>[4x]RHMQEILDAILSGDAASADYAALALPESYRAVTLHKGEERMFDGLASRDKDPRKSLHLDDVPLPELGPGEALVAVMASSVN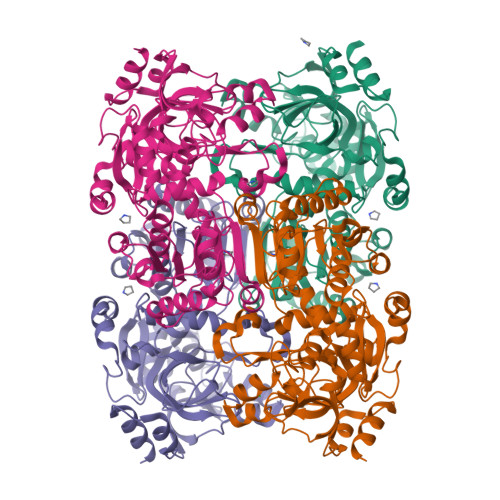YNTVWSSIFEPVSTFGFLERYGRLSPLTARHDLPYHVLGSDLAGVVLRTGAGVNAWKPGDEVVAHCLSVELESPDGHNDTMMDPEQRIWGFETNFGGLAQLALVKTNQLLPKPKHLTWEEAASPGLVNSTAYRQLVSRNGAGLKQGDNVLIWGASGGLGSYATQYALAGGATPICVVSSPRKADICRAMGAEAIIDRSAEGYRFWKDEHHQDPREWKRLGGKIREFTGGEDVDIVFEHPGRETFGASVYVTRKGGTIVTCASTSGYMHQYDNRYLWMSLKRIVGSHFANYREAFEANRLVAKGKIHPTLSKVYALEETGQAALDVHHNKHQGKVGVLCLAPREGLGVTDPELRSKHLTKINAFR>MSLDNLDVICIGAAIVDIPLQPVSKNIFDVDSYPLERIAMTTGGDAINEATIISRLGHRTALMSRIGKDAAGQFILDHCRKENIDIQSLKQDVSIDTSINVGLVTEDGERTFVTNRNGSLWKLNIDDVDFARFSQAKLLSLASIFNSPLLDGKALTEIFTQAKARQMIICADMIKPRLNETLDDICEALSYVDYLFPNFAEAKLLTGKETLDEIADCFLACGVKTVVIKTGKDGCFIKRGDMTMKVPAVAGITAIDTIGAGDNFASGFIAALLEGKNLRECARFANATAAISVLS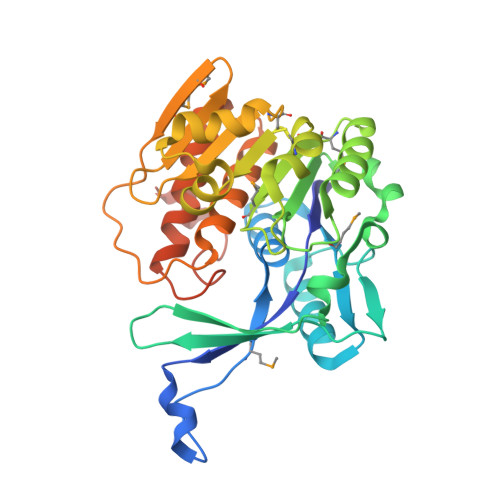VGATTGVKNRKLVEQLLEEYEGEGHHHHHH[2x]>HPETLVKVKDAEDQLGARVGYIELDLNSGKILESFRPEERFPMMSTFKVLLCGAVLSRIDAGQEQLGRRIHYSQNDLVEYSPVTEKHLTDGMTVRELCSAAITMSDNTAANLLLTTIGGPKELTAFLHNMGDHVTRLDRWEPELNEAIPNDERDTTMPVAMATTLRKLLTGELLTLASRQQLIDWMEADKVAGPLLRSALPAGWFIADKSGAGERGSRGIIAALGPDGKPSRIVVIYTTGSQATMDERNRQIAEIGASLIKHW[2x];>[2x]AGVMTGAKFTQIQF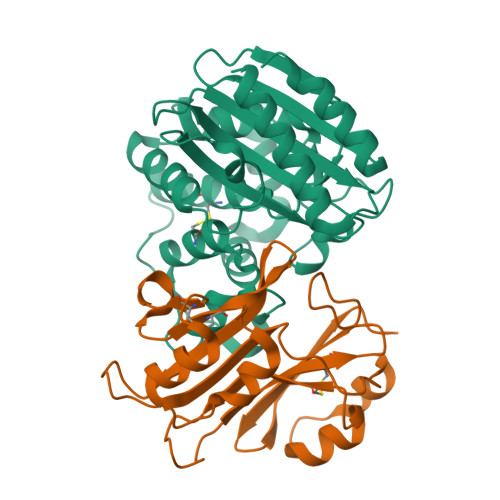GMTRQQVLDIAGAENCETGGSFGDSIHCRGHAAGDYAAYATFGFTSAAADAKVDSKSQEKLLAPSAPTLTLAKFNQVTVGMTRAQVLATVGQGSCTTWSEYYPAYPSTAGVTLSLSCFDVDGYSSTGFYRGSAHLWFTDGVLQGKRQWDLV> MELIQDTSRPPLEYVKGVPLIKYFAEALGPLQSFQARPDDLLINTYPKSGTTWVSQILDMIYQGGDLEKCNRAPIYVRVPFLEVNDPGEPSGLETLKDTPPPRLIKSHLPLAL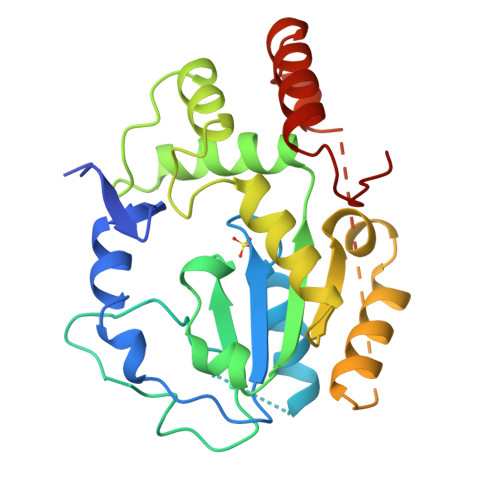LPQTLLDQKVKVVYVARNPKDVAVSYYHFHRMEKAHPEPGTWDSFLEKFMAGEVSYGSWYQHVQEWWELSRTHPVLYLFYEDMKENPKREIQKILEFVGRSLPEETMDFMVQHTSFKEMKKNPMTNYTTVPQELMDHSISPFMRKGMAGDWKTTFTVAQNERFDADYAEKMAGCSLSFRSEL>[2x]SNAMKKWIYVVLVLSIAGIGGFSVHAASSAHEKHLNVSKMNVDDEFKDT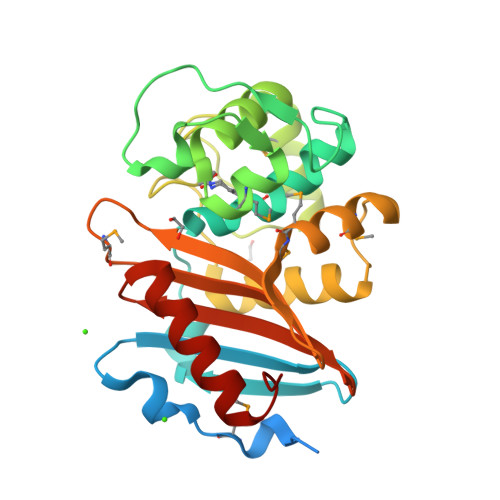DGTFILHDLQKDQTFVYNRKRANQRQTPQSTFKVVNALIGLQVKAVRDEYDVKRWDGVKREFESWNRDHTLGSAMRESAIWYYQALARDIGEERMKTWLHTLSYGNEDISGGIDQFWLQSSLTISPLEQETFLEKLAKEELPFDKPVMKIVKRMMIQEEGDHYTLYGKTGTRLTDMGLGWFVGFIKTEHGSYVFVTNVDDSGTKAKNITVDILKKYGLITS> MPNTSQRNSFLQDVPYWMLQNRSEYITQGVDSSHIVDGKKTEEIEKIATKRATIRVAQNIVHKLKEAYLSKTNRIKQKITNEMFIQMTQPIYDSLMNVDRLGIYINPNNEEVFALVRARGFDKDALSEGLHKMSLDNQAVSILVAKVE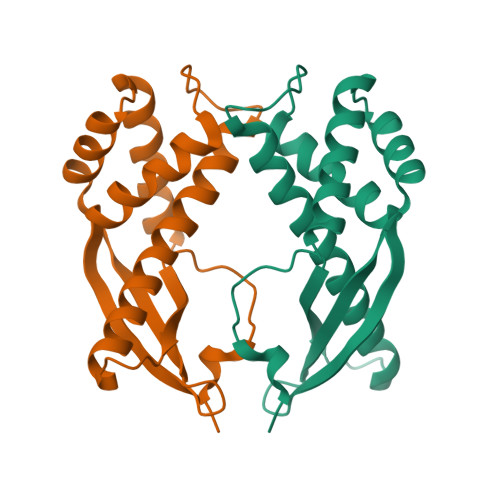EIFKDSVNYGDVKVPIAM> GSMYQLQFINLVYDTTKLTHLEQTNINLFIGNWSNHQLQKSICIRHGDDTSHNQYHILFIDTAHQRIKFSSFDNEEIIYI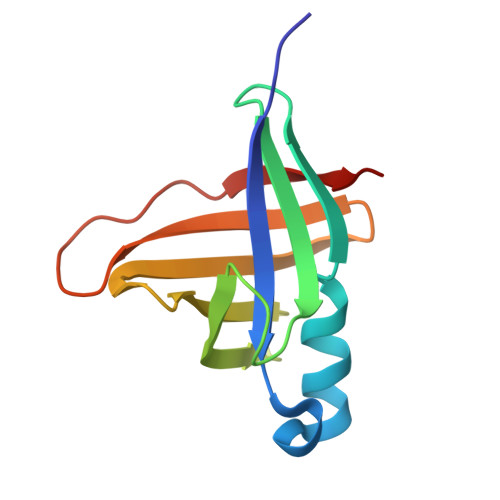LDYDDTQHILMQTSSKQGIGTSRPIVYERLV>[2x]MLRFAVLGHPVAHSLSPAMHAFALESLGLEGSYEAWDTPLEALPGRLKEVRRAFRGVNLTLPLKEAALAHLDWVSPEAQRIGAVNTVLQVEGRLFGFNTDAPGFLEALKAGGIPLKGPALVLGAGGAGRAVAFALREAGLEVWVWNRTPQRALALAEEFGLRAVPLEKAREARLLVNATRVGLEDPSASPLPAELFPEEGAAVDLVYRPLWTRFLREAKAKGLKV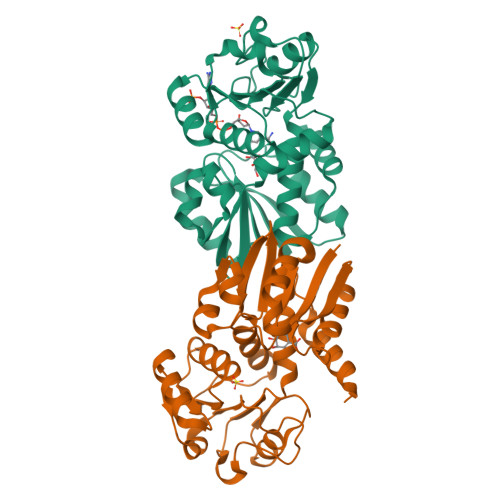QTGLPMLAWQGALAFRLWTGLLPDPSGMEEAARRALGV MONO-{4-[(4-AMINO-2-METHYL-PYRIMIDIN-5-YLMETHYL)-AMINO]-2-HYDROXY-3-MERCAPTO-PENT-3-ENYL-PHOSPHONO} ESTER | C11 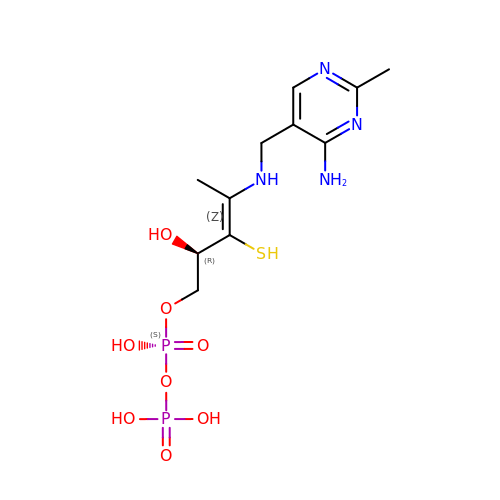H20 N4 O8 P2 S | XHCFSNVIKLFNIT-WPVMNKCKSA-N> MSAPNPKAFPLADAALTQQILDVVQQAANLRQLKKGANEATKTLNRGISEFIIMAADCEPIEILLHL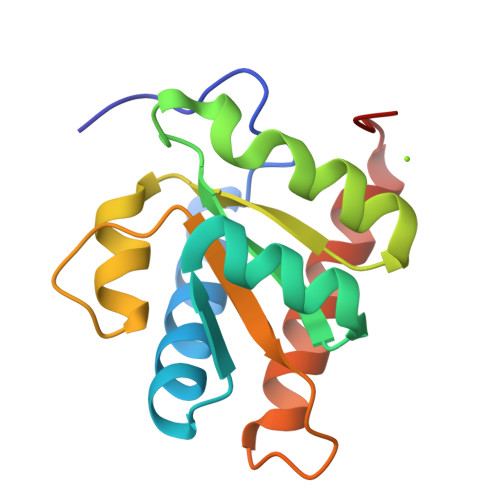PLLCEDKNVPYVFVPSRVALGRACGVSRPVIAASITTNDASAIKTQIYAVKDKIETLLILEHHHHHH>[4x]MLPPLPDFSLSVEQQFDLQKYRQQVRDISREDLEDLFIEVVRQKMAHENIF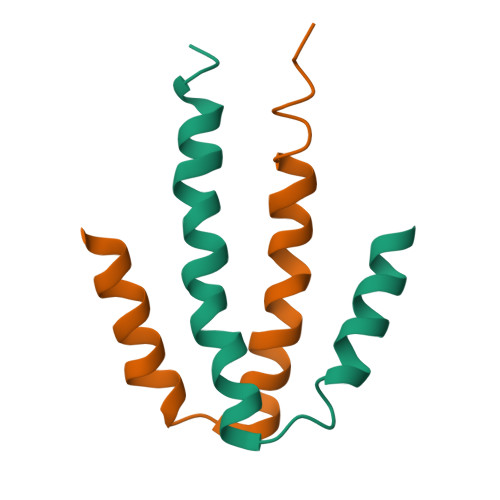KGMIRQGS> I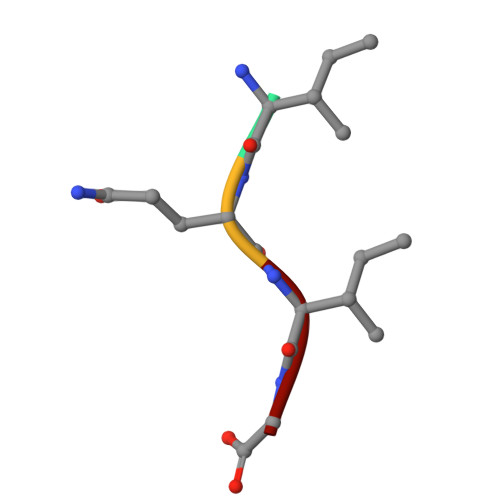QIG> MAHHHHHHHRSSGTDAGTAGTAGTAGAGAGGDRQHVDALVRMSNLVTPMALRVAATLRLVDHLRAGATSADALADATGADADALARLMRHLAAAGVLEEPEPGHYAPTGLGDLLADDHPSRQRSWLDLDQAVGRADLTFLGLREAVRTGRPQYEARYGKPFWTDLSEDDGLGASFDALMTTREDTAFAAPVAAYDWTRARHVLDVGGAPGGLLTAILRAAPEAHGTLLDLPGAAARTRERIAANGMDERIDVVGGDFFDELPVTADVVVLSFTLLNWSDPDALRILGRCRDALRPGGRIVLLERAEAPSGGTRTSDLYFSVLDMRMLVFLGGRVRTDREWADLAAAAGLDIVGKTGPL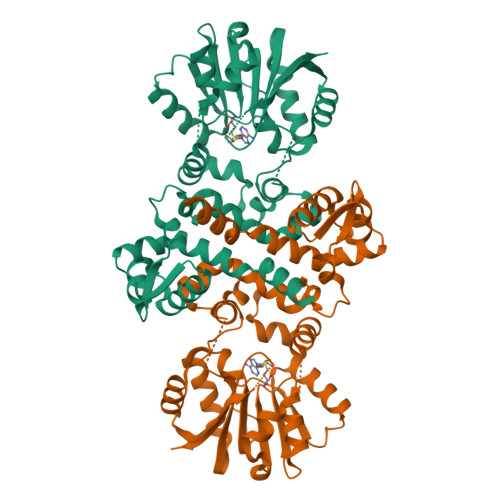VSPNVPLDSCLWELAPR> QSNAMRLPYSWLREVVAVGASGWDVTPGELEQTLLRIGHEVEEVIPLGPVDGPVTVGRVADIEELTGYKKPIRACAVDIGDRQYREIICGATNFAVGDLVVVALPGATLPGGFTISARKAYGRNSDGMICSAAELNLGADHSGILVLPPGAAEPGADGAGVLGLDDVVFHLAITPDRGYCMSVRGLARELACAYDLDFVDPASNSRVPPLPIEGPAWPLTVQPETGVRRFALRPVIGIDPAAVSPWWLQRRLLLCGIRATCPAVDVTNYVMLELGHPMHAHDRNRISGTLGVRFARSGETAVTLDGIERKLDTADVLIVDDAATAAIGGVMGAASTEVRADSTDVLLEAAIWDPAAVSRTQRRLHLPSEAARRYERTVDPAISVAALDRCARLLADIAGGEVSPTLTDWRGDPPCDDWSPPPIRMGVDVPDRIAGVAYPQGTTARRLAQIGAVVTHDGDTLTVTPPSWRPDLRQPADLVEEVLRLEGLEVIPSVLPPAPAGRGLTAGQQRRRTIGRSLALSGYVEILPTPFLPAGVFDLWGLEADDSRRMTTRVLNPLEADRPQLATTLLPALLEALVRNVSRGLVDVALFAIAQVVQPTEQTRGVGLIPVDRRPTDDEIAMLDASLPR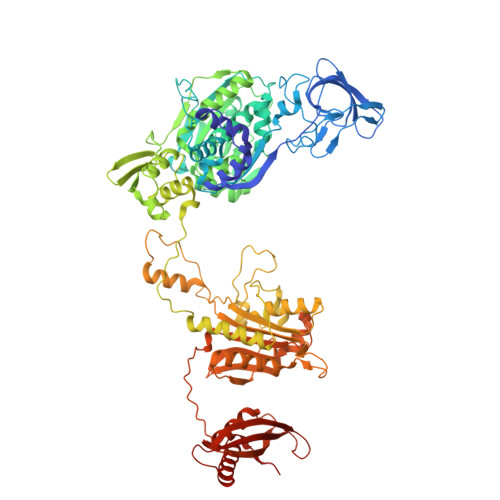QPQHVAAVLAGLREPRGPWGPGRPVEAADAFEAVRIIARASRVDVTLRPAQYLPWHPGRCAQVFVGESSVGHAGQLHPAVIERSGLPKGTCAVELNLDAIPCSAPLPAPRVSPYPAVFQDVSLVVAADIPAQAVADAVRAGAGDLLEDIALFDVFTGPQIGEHRKSLTFALRFRAPDRTLTEDDASAARDAAVQSAAERVGAVLRG> MEHVAFGSED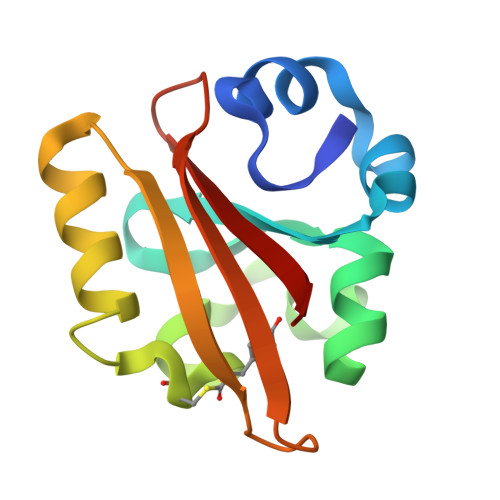IENTLAKMDDGQLDGLAFGAIQLDGDGNILQYNAAESDITGRDPKQVIGKNFFKDVAPCTDSPEFYGKFKEGVASGNLNTMFEYTFDYQMTPTKVKVHMKKALSGDSYWVFVKRV>[2x]CG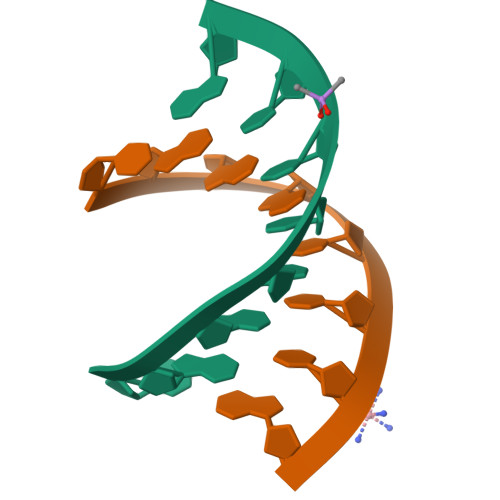AAXUCG> GPMTTTERPDLAWLDEVTMTQLERNPYEVYERLRAEAPLAFVPVLGSYVASTAEVCREVATSPDFEAVITPAGGRTFGHPAIIGVNGDIHADLRSMVEPALQPAEVDRWIDDLVRPIARRYLERFENDGHAELVAQYCEPVSVRSLGDLLGLQEVDSDKLREWFAKLNRSITNAAVDENGEFANPEGFAEGDQAKAEIRAVVDPLIDKWIEHPDDSAISHWLHDGMPPGQTRDREYIYPTIYVYLLGAMQEPGHGMASTLVGLFSRPEQLEEVVDDPTLIPRAIAEGLRWTSPIWSATARISTKPVTIAGVDLPAGTPVMLSYGSANHDTGKYEAPSQYDLHRPPLPHLAFGAGNHACAGIYFANHVMRIALEELFEAIPNLERDTREGVEFWGWGFRGPTSLHVTWEV

GcoA belongs to the CYP255A family of cytochrome P450 enzymes. Our recent characterization of a two-component P450 enzyme system consisting of a reductase, GcoB, and a P450 oxidase, GcoA, demonstrated that it demethylates diverse aromatic compounds, including guaiacol (which can be derived from coniferyl alcohol and represents the aromatic functionality of G-lignin that must undergo demethylation), guaethol, anisole (methoxybenzene), 2-methylanisole, and 3-methoxycatechol (3MC) with similar or greater efficiency than other O-aryl-demethylases described in the literature. However, GcoAB shows poor reactivity toward syringol, which can be derived from sinapyl alcohol via high-temperature reactions and represents the aromatic functionality of S-lignin that must undergo O-demethylation for further catabolism via ring-opening dioxygenases. In the present study, we hypothesized that substitution of GcoA-F169, which has the closest interaction with the bound substrate, may relax the specificity of the enzyme sufficiently to permit the O-demethylation of S-lignin type substrates.

The closest contact is with GcoA-F169, which forms a hydrophobic interaction with the C6 carbon on the aromatic ring of guaiacol. A broader survey of variants at the GcoA-F169 position (amino acids S, H, V, I, and L in addition to A) confirmed that GcoA-F169A exhibits the best catalytic performance in terms of both specific activity and reaction coupling, although other small side chains (S and V) also permitted reactivity with syringol, suggesting that these may permit syringol to assume a reactive conformation at the heme. Each protein variant also crystallized successfully with guaiacol and the structures showed that the orientation of the bound ligand remained consistent with that of the WT enzyme. Furthermore, comparison of the surrounding active site architecture confirmed no significant deviation from the WT.2-oxoheptanedioic acid | C7 H10 O5 | 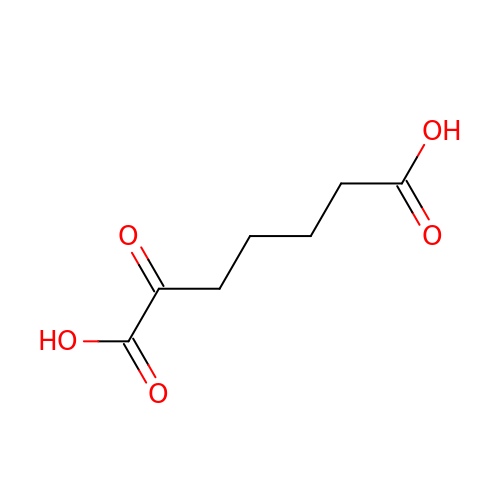HABHUTWTLGRDDU-UHFFFAOYSA-N>[2x]MAHHHHHHMKIAVLPGDGIGPEIVNEAVKVLNALDEKFELEHAPVGGAGYEASGHPLPDATLALAKEADAILFGAVGDWKYDSLERALRPEQAILGLRKHLELFANFRPAICYPQLVDASPLKPELVAGLDILIVRELNGDIYFGQPRGVRAAPDGPFAGEREGFDTMRYSEPEVRRIAHVAFQAAQKRAKKLLSVDKSNVLETSQFWRDVMIDVSKEYADVELS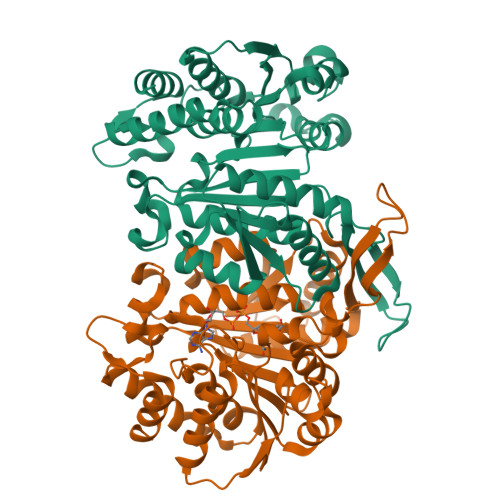HMYVDNAAMQLAKAPKQFDVIVTGNMFGDILSDEASMLTGSIGMLPSASLDKNNKGLYEPSHGSAPDIAGKGIANPLATILSAAMLLRYSLNRAEQADRIERAVKTVLEQGYRTGDIATPGCRQVGTAAMGDAVVAAL The sodium-driven chloride/bicarbonate exchanger (NDCBE) is a member of the sodium-bicarbonate cotransporters (NBCs) within the solute carrier 4 (SLC4) gene family. In the brain, NDCBE is primarily associated with the presynaptic vesicles of glutamatergic and GABAergic neurons. In the plasma membrane, most SLC4 transporters are believed to form functional dimers. Furthermore, NDCBE activity depends on a Na+ gradient.

Here, we present the crystal structure of the truncated (ΔVR1, residues 1–39) N-terminal cytoplasmic domain from human NDCBE-D (ntcNDCBE) at 2.8 Å resolution. Each monomeric ntcNDCBE forms an α-β sandwich fold by nine α-helices and ten β-strands. The main dimer interface is generated through a domain-swapped antiparallel β-sheet, including β-strands 5 and 10. The domain-swapped β-sheet is stabilized by backbone hydrogen-bonding interactions between residues Thr341 and Leu343 from β10 in each monomer, as well as backbone hydrogen bonds by Leu108 (β5) with Val342 (β10) and Leu110 (β5) with Val340 (loop between α9 and β10) on the adjacent sides. However, to establish whether ntcNDCBE forms a dimer in solution at lower concentrations, the construct was subjected to size-exclusion chromatography (SEC), and eluted at volumes corresponding to the hydrodynamic volume of a dimer. By superimposing the central β-sheet (β1-3, β6-9) of the individual monomers of cdb3 (chain P) and ntcNDCBE (chain A), a pivotal movement of ~23° is observed between each monomer, while the central dimerization domain-swapped β-sheet (β5, β10) remains intact. We identify and describe a novel Zn2+-binding site and the completely conserved HHH motif also found in the electroneutral sodium-bicarbonate transporters (NBCn1 and NCBE) surrounded by a shell of negatively charged residues on the surface of ntcNDCBE. In the WT protein, Trp80 is engaged in a π-π stacking with His167, which is likely rearranged upon Zn2+ binding. The experiments were severely hampered by the crystal conditions, as we were only able to form crystals at pH 4.4.

>[2x]MPLGRQSHRHHRTHGQKHRRRGRGKGASQGEEGLEALAHDTPSQRVQFILGTEEDEEHVPHELFTELDEICMKEGEDAEWKETARWLKFEEDVEDGGERWSKPYVATLSLHSLFELRSCLINGTVLLDMHANSIEEISDLILDQQELSSDLNDSMRVKVREALLKKHHHQNEKKRNNLIPIVRSFAEVGKKQSDPHLMDKHGQTVSPQSVPTTNLEVKNGVNCEHSPVDLSKVDLHFMKKIPTGAEASNVLVGEVDILDRPIVAFVRLSPAVLLSGLTEVPIPTRFLFILLGPVGKGQQYHEIGRSMATIMTDEIFHDVAYKAKERDDLLAGIDEFLDQVTVLP>[2x]GSHMGTDTDE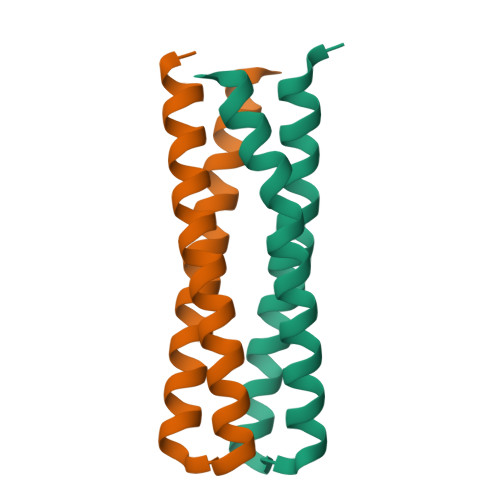LLRLAKEQAELLKEIKKLVEEIARLVKEIQEDPSDELLKTLAELVRKLKELVEDMERSMKEQLYIIKKQKS> MGYYDDDGNYHSFRRGVERAVDRITHPFHHHHHHHDREEVVIADERGPVRYRDGVREDVRIVEPRASKTTAESVPIPCHFIRIGDILILQGRPCQVIRISVSPQTGQHRYLGVDLFTRQLQEESSFVSNPSPSVVVQTMLGPVYKT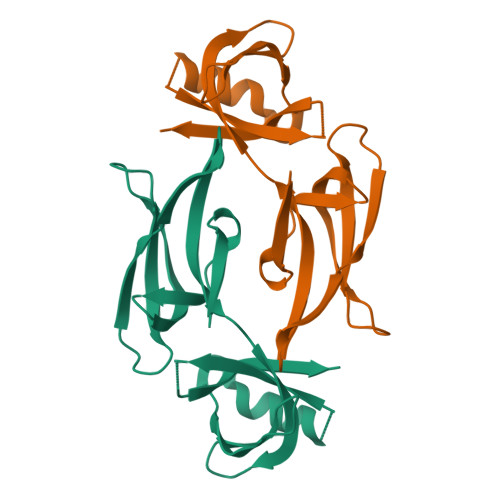YRILDLHEDGTITAMTETGDVKQALPVVTQGQLFRKIRDAFSEGRGSVRALVINDGGRELVVDYKVIHGSRL>MKTVVFAYHDMGCLGIEALLAAGYEISAIFTHTDNPGEKAFYGSVARLAAERGIPVYAPDNVNHPLWVERIAQLSPDVIFSFYYRHLIYDEILQLAPAGAFNLHGSLLPKYRGRAPLNWVLVNGETETGVTLHRMVKRADAGAIVAQLRIAIAPDDIAITLHHKLCHAARQLLEQTLPAIKHGNILEIAQRENEATCFGRRTPDDSFLEWHKPASVLHNMVRAVADPWPGAFSYVGNQKFTVWSSRVHPHASKAQPGSVISVAPLLIACGDGALEIVTGQAGDGITMQGSQLAQTLGLVQ[4x];>MRVLILGVNGFIGNHLTERLLREDHYEVYGLDIGSDAISRFLNHPHFHFVEGDISIHSEWIEYHVKKCDVVLPLVAIATPIEYTRNPLRVFELDFEENLRIIRYCVKYRKRIIFPSTSEVYGMCSDKYFDEDHSNLIVGPVNKPRWIYSVSKQLLDRVIWAYGEKEGLQFTLFRPFNWMGPRLDNLNAARIGSSRAITQLILNLVEGSPIKLIDGGKQKRCFTDIRDGIEALYRIIENAGNRCDGEIINIGNPENEASIEELGEMLLASFEKHP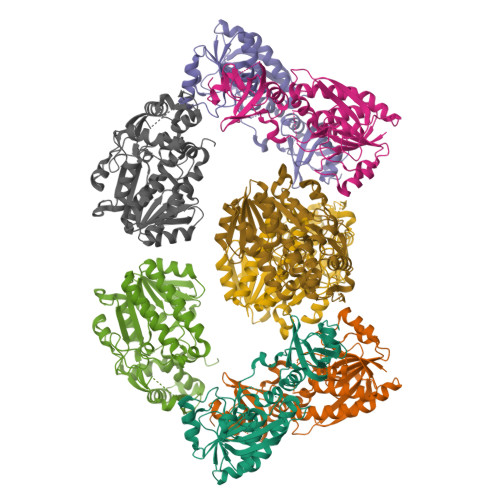LRHHFPPFAGFRVVESSSYYGKGYQDVEHRKPSIRNAHRCLDWEPKIDMQETIDETLDFFLRTVDLTDKPS[4x]>[2x]YVEFMSTNTKHYDYLVIGGGSGGVASARRAASYGAKTLLVEAKALGGTCVNVGCVPKKVMWYASDLATRVSHANEYGLYQNLPLDKEHLTFNWPEFKQKRDAYVHRLNGIYQKNLEKEKVDVVFGWARFNKDGNVEVQKRDNTTEVYSANHILVATGGKAIFPENIPGFELGTDSDGFFRLEEQPKKVV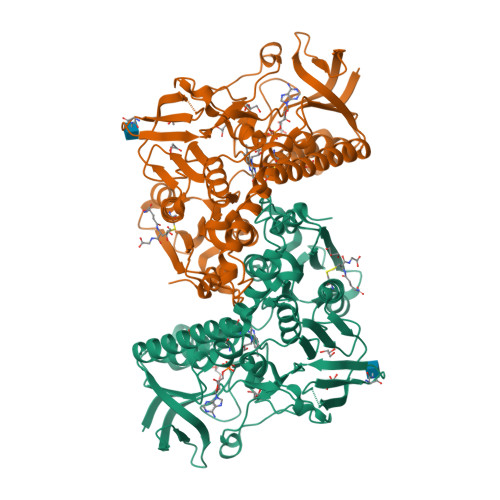VVGAGYIGIELAGVFHGLGSETHLVIRGETVLRKFDECIQNTITDHYVKEGINVHKLSKIVKVEKNVETDKLKIHMNDSKSIDDVDELIWTIGRKSHLGMGSENVGIKLNSHDQIIADEYQNTNVPNIYSLGDVVGKVELTPVAIAAGRKLSNRLFGPEKFRNDKLDYENVPSVIFSHPEAGSIGISEKEAIEKYGKENIKVYNSKFTAMYYAMLSEKSPTRYKIVCAGPNEKVVGLHIVGDSSAEILQGFGVAIKMGATKADFDNCVAIHPTSAEELVTMRGSHHHHHH>[6x]MFQRSIPALITPFTKDNLIDEDSFVDHIEWQISEGSSGLVPAGTTGESSTLSYEEHCRVVELCVKTAAGRVPVMAGAGSNNTKESIELAQYAQNTGADALLVVVPYYNKPNKKGLLAHFGSIANAVSLPIYIYNNPSRTVIEMDVDTMA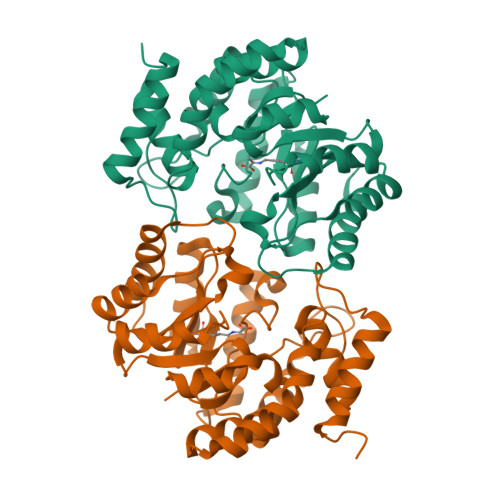ELVKTYSNIVGVKDATGRIELASGQRIACGSDFIQLSGDDSSALGFNVHGGVGCISVTANVAPRICAEFQKAISEGDYRQALEYQDKLFPLHQALFIEPSISSVKYALSRLGRNVSLVVRAPMVSILEKETMFAIDQALDHIGLCA> GPMRRSYEGYKVYGIVPESPDEAEILYQIRQSNPDLDFWHLTKQPGDEARVLVAP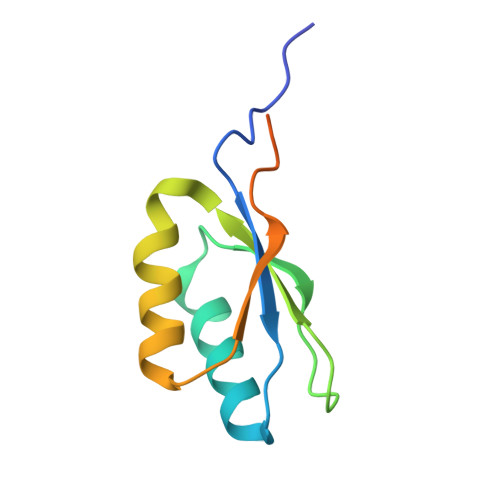KDQRSFLIKLIRHGLHYQEVISDVEGTLAPYNEPRTRGMSLDR ChRmine is a bacteriorhodopsin-like cation channelrhodopsin (BCCR) more closely related to ion pump rhodopsins than other channelrhodopsins. ChRmine displays unique properties favorable for optogenetics including high light sensitivity, a broad, red-shifted activation spectrum, cation selectivity, and large photocurrents, while its slow closing kinetics impedes some applications. ChRmine is a homotrimer with a central pore between subunits, unlike all other channelrhodopsins of known structure which are homodimers. The general topology of each ChRmine subunit is typical of rhodopsins, with an extracellular N-terminal region (amino acids 2–26), seven transmembrane helices (TM1-7, amino acids 27–270), intracellular and extracellular linkers (ICL1-3 and ECL1-3), a cytoplasmic C-terminal region.

We observed two populations of ChRmine particles distinguished by nanodisc diameter. Particles with small and large diameter nanodiscs were processed separately and generated reconstructions to 2.7 Å and 3.1 Å resolution, respectively. The cytoplasmic C-terminal 19 amino acids are not visible in the cryo-EM map, likely due to disorder. Both maps display clear density for one retinal and multiple lipids per subunit, while the higher resolution map from small diameter ChRmine nanodiscs showed additional density for nineteen ordered water molecules per subunit. As there are no other substantial differences between the two ATR-bound ChRmine structures (overall r.m.s.d. = 0.28 Å), we focus our discussion below on the higher resolution structure unless otherwise noted. A conserved lysine (K257) on TM7 is covalently linked to a molecule of all-trans retinal through a Schiff base. As expected, the channel is captured in a closed ground state conformation, but the relative positions of TM1, TM2, TM3, and TM7 create deep extracellular and intracellular cavities for ion conduction that are only sealed from one another at the Schiff base. However, the intracellular central cavity is nonpolar and packed with lipids that preclude ion passage. Consistent with the nonpolar environment (and analogous to ion pump rhodopsin trimers), we observe strong tube-shaped features in this region that are well fit by three complete and tightly packed DOPE lipid molecules. Association of lipid acyl chains results in constrictions less than 1 Å in radius, effectively sealing the pore. We conclude the central pore is unlikely to serve as a conduction pathway in ChRmine.

>MAHAPGTDQMFYVGTMDGWYLDTKLNSVAIGAHWSCFIVLTITTFYLGYESWTSRGPSKRTSFYAGYQEEQNLALFVNFFAMLSYFGKIVADTLGHNFGDVGPFIIGFGNYRYADYMLTCPMLVYDLLYQLRAPYRVSCSAIIFAILMSGVLAEFYAEGDPRLRNGAYAWYGFGCFWFIFAYSIVMSIVAKQYSRLAQLAQDTGAEHSLHVLKFAVFTFSMLWILFPLVWAICPRGFGWIDDNWTEVAHCVCDIVAKSCYGFALARFRKTYDEELFRLLEQLGHDEDEFQKLELDMRLSSNGERLRRLSLNSLEVLFQ[3x]>MDIISVALKRHSTKAFDASKKLTPEQAEQIKTLLQYSPSSQNSQPWHFIVASTEEGKARVAKSAAGNYVFSERKMLDASHVVVFCAKTAMDDVWLKLVVDQEDADGRFATPEAKAANDKGRKFTADVHRKDLHDDAEWMAKQVYLNVGNFLLGVAALGLDAVPIEGFDAAILDAEFGLKEKGYTSLVVVPVGHHSVEDFNATLPKSRLPQNITLTEV[2x]

Escherichia coli NfsB has been studied extensively for its potential for cancer gene therapy by reducing the prodrug CB1954 to a cytotoxic derivative. The natural substrate of this flavoprotein enzyme is not known; however, it reduces a wide range of nitroaromatic compounds to hydroxylamines and also reduces quinones to quinols, with a bi-bi substituted (ping-pong) enzyme mechanism. The enzyme is a homodimer of two 24 kDa subunits with an extensive dimer interface. The two active sites are on opposite sides of the long central helix at the dimer interface, and the FMN is bound to residues from both monomers.

Our most active mutant in E. coli is T41Q/N71S/F124T/M127V, in which the additional M127V mutation enlarges the small channel to the active site. The structure of this mutant was determined at 2 Å resolution. The side chain change of this additional mutation is too far away to have a direct effect on the active site of NfsB; however, the M127V mutation enlarges a small channel leading to the active site. In NfsB, the main opening to the active site is as shown in Figure 1; however, there is a smaller opening to the site, approximately at right angles to the first one, shown in Figure 7. In the wild-type protein, a protein bridge, formed by F124 and Y68 side chains, is above this small channel so that it is only large enough for solvent and small ions. In the triple mutant, two smaller bridges form between M127 and Y68 and between N67 and F123. However, the mutation of M127 to the smaller valine allows the side chains of Y68 and N67 to move slightly, opening the channel. This could allow larger substrates to be accommodated in the active site. The steady-state kinetics of reduction of CB1954 with the T41Q/N71S/F124T/M127V mutant shows the highest kcat of all the mutants to date and a much lower Km for CB1954 than the wild-type enzyme, so it should be much more active with the prodrug. The quadruple mutant has the highest activity in the colony-forming assays in E. coli, with about a fifty-fold increase in sensitivity to CB1954 over the wild-type enzyme, similar in magnitude to its decrease in Km for CB1954.> MADDQWVPDVPDGAFVIGGGDYRYGQDMTEDIARSLFQVPDFNPANALLVLPQLLLRLPLEALQKFKDFIPNVLEGAFNTVA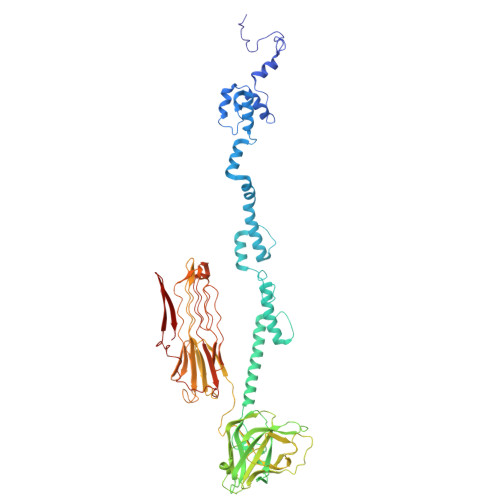GAVDAIMGAIRETPRVLEQILSYLPQELRDELEHAAARIGAVIDAIVQALTGTLNIGHTIEDLIFSLTNIRPGAVGGVLGGGSIEETIKRIVDAIVSGIVGVTGIGAGISDLQSLIEQISSAAARGGFAWDILGIQNNKKPKSGLYKSERGNFDLDTLNSTVSVAPGTSIIAFDVIEQSMPIGLITWIGWGTSGITEFYINVYRCVDDRSDPELGELIHQSENIAGLLAGSASPGANMAYELTTPIEAVAGDLLAYEFIAVGGTHTMRGRDFNLPDNDGAPIGNVGATRSLSTPSLPPATLDKADVTWTDNVPRVGIAVDTGTGSDHHDPQVEFFEKPVAIPVPAWCDRIDAIVTGKGGEGADGFLGFYGNPGQPGSVNTVTWTRGEHFSGTTTILEWDGAELSIPGFEVSAANGSNGSGQRPVALGKPVGKGIEEVEYNGLKLAAGGDQHAYGGAGTKPGGGGNGGHWLGIYTQGGPGGPACAAVQFRKGALPGEVVGDGEGDVTPPNVSALHVDVSATSTSITITPSGAVDDA>[4x]GSHMASGEGPALYEDPPDQKTSPSGKPATLK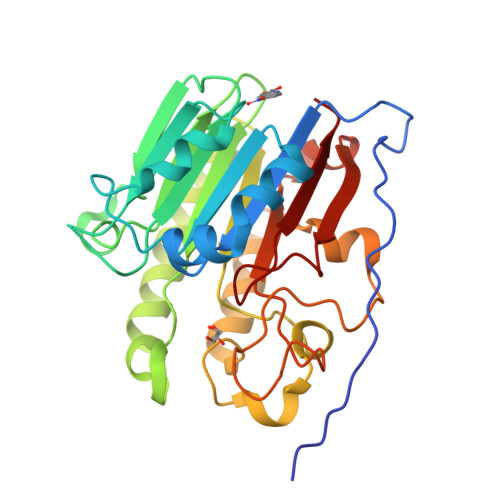ICSWNVDGLRAWIKKKGLDWVKEEAPDILCLQETKCSENKLPAELQELPGLSHQYWSAPSDKEGYSGVGLLSRQCPLKVSYGIGDEEHDQEGRVIVAEFDSFVLVTAYVPNAGRGLVRLEYRQRWDEAFRKFLKGLASRKPLVLCGDLNVAHEEIDLRNPKGNKKNAGFTPQERQGFGELLQAVPLADSFRHLYPNTPYAYTFWTYMMNARSKNVGWRLDYFLLSHSLLPALCDSKIRSKALGSDHCPITLYLAL>LVAEDAPVLSKAFVDRVNRLNRGIWKAKYDGVMQNITLREAKRLNGVIKKNNNASILPKRRFTEEEARAPLPSSFDSAEAWPNCPTIPQIADQSACGSCWAVAAASAMSDRFCTMGGVQDVHISAGDLLA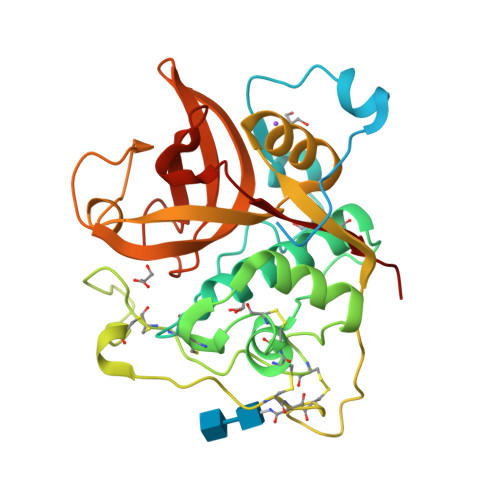CCSDCGDGCNGGDPDRAWAYFSSTGLVSDYCQPYPFPHCSHHSKSKNGYPPCSQFNFDTPKCNYTCDDPTIPVVNYRSWTSYALQGEDDYMRELFFRGPFEVAFDVYEDFIAYNSGVYHHVSGQYLGGHAVRLVGWGTSNGVPYWKIANSWNTEWGMDGYFLIRRGSSECGIEDGGSAGIPLAPNTA[2x]> ADLVPPPGYYAAVGERKGSAGSCPAVPPPYTGSLVFTSKYEGSDSARATLNVKAEKTFRSQIKDITDMERGATKLVTQYMRSGRDGDLACALNWMSAWARAGALQSDDFNHTGKSMRKWALGSLSGAYMRLKFSSSRPLAAHA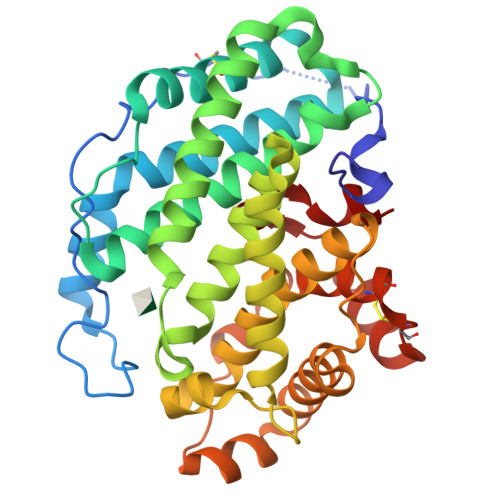EQSREIEDWFARLGTQVVRDWSGLPLKKINNHSYWAAWSVMSTAVVTNRRDLFDWAVSEFKVAANQVDEQGFLPNELKRRQRALAYHNYALPPLAMIAAFAQVNGVDLRQENHGALQRLAERVMKGVDDEETFEEKTGEDQDMTDLKVDNKYAWLEPYCALYRCEPKMLEAKKDREPFNSFRLGGEVTRVFS MALONYL-COENZYME A | C24 H38 N7 O19 P3 S | 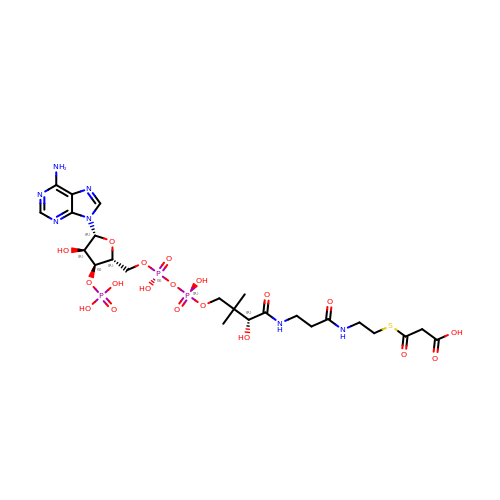LTYOQGRJFJAKNA-DVVLENMVSA-N N-[(4S,8E,11S)-4-[(1R)-1-hydroxy-2-{[3-(propan-2-yl)benzyl]amino}ethyl]-2,13-dioxo-11-phenyl-6-oxa-3,12-diazabicyclo[12.3.1]octadeca-1(18),8,14,16-tetraen-16-yl]-N-methylmethanesulfonamide 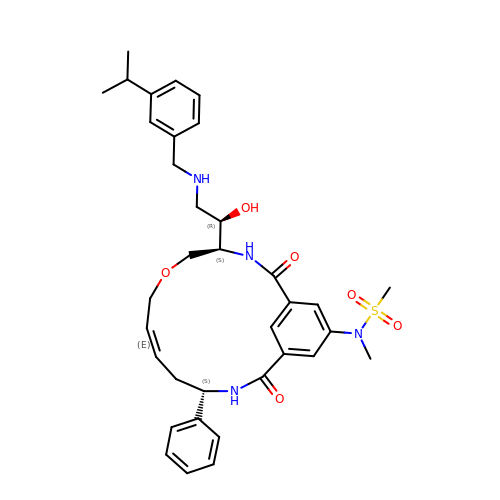| C35 H44 N4 O6 S | XYJDOUBLYLOJJL-YNYOQIOBSA-N> MVDINLFREEKGNNPEIIRESQ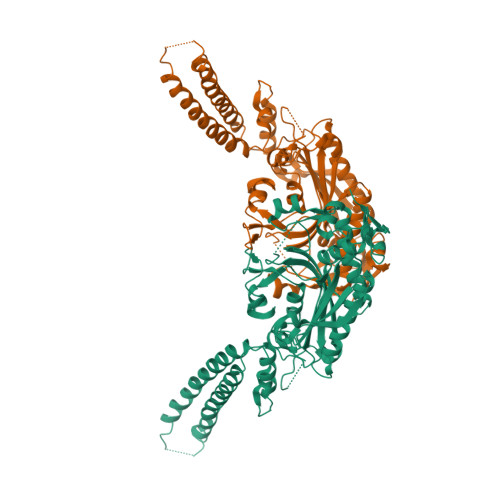RRRFASVEIVDEIIKLDKEWRQRQFEVDSFRKEFNKLNKQVAQLKIKKEDASEIIQQTEKNKQDSTAKEAEVREAYAALKAKLEQVGNLVHDSVPVDKDEANNLVIKLWGEKRFSTPGLKLKNHVDLVELLGIADTKRGAEIAGARGFFLKGDGLMLNQALINFGLTFLKKRGFTGLQPPFFMRKDVMAKCAQLAQFDEELYKVTGEGDDKYLIATAEQPLSAYHIDEWIHPTELPLRYAGYSSCFRKEAGSHGRDTLGIFRVHQFEKIEQFCITGPNENASWEMLDEMMKNSEDFYQALKLPYQIVSIVSGALNDAAAKKYDLEAWFPSSETFRELVSCSNCTDYQARRLEIRYGQKKSNEQTKQYVHMLNSTLTATERTICCILENYQREDGVDIPEVLQPFMGGETFLPFKAKPVVADTKGKKSKAAAALE>MGIQVIATTPFKDQKPGTSGLRKPVPVFQQPHYLENFIQAIFDTIEAPQGQTLVLGGDGRYFNAEAIQVILKMAAAKGFARVKVGQNGILSTPAASCVIRKYGAVGGIILSASHNPAGPQGDFGVKFNIANGGPAPEKVTNAIYERSLALTHYSIYTAPDVNLHTLGEFPLGEMIVEVIDPVADYQALLETLFDFDRIAEVIRTGKLRLVFDAMHAVTGPYAQQILEKCLGAPPGTVQNGVPLPDFGGGHPDPNLVYAHDLVQQLFGEQPPDFGAASDGDGDRNMILGANCFVTPSDSLAILAANAQLVPGYRDGLAGIARSMPTSQAADRVAAKLGIDCYETPTGWKFFGNLLDAGKVTLCGEESFGTGSNHVREKDGLWAVLFWLNILAVRQTPVAEIVKDHWRTYGRNYYSRHDYEGIEGDRAHTLMSQLEQKLPSLVGQTLGAYTVATADNFSYSDPVDHSVSQNQGIRLIFEDGSRIVYRLSGTGTQGATLRVYLERFEPHPSQQHLDAQVALADLIQLA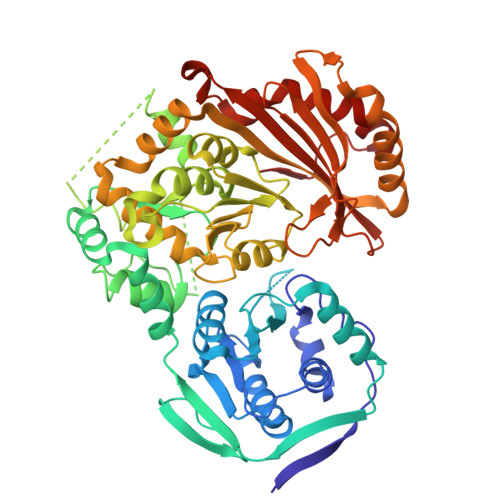NDVANIQSLTGRDRPTVIT[2x]> GSNLVAQLENEVASLENENETLKK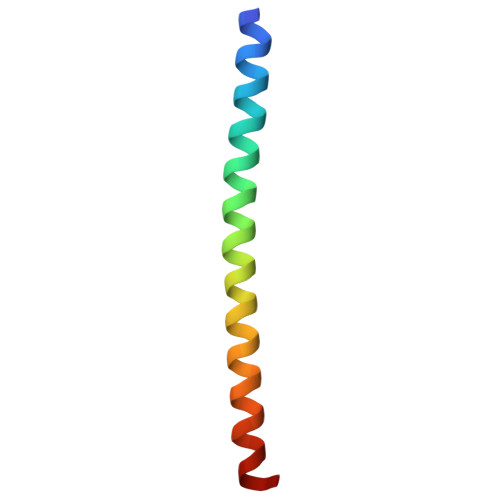KNLHKKDLIAYLEKEIANLRKKIEE> SMEMYETLGKVGEGSYGTVMKCKHKNTGQIVAIKIFYERPEQSVNKIAMREIKFLKQFHHENLVNLIEVFRQKKKIHLVFEFIDHTVLDELQHYCHGLESKRLRKYLFQILRAIDYLHSNNIIHRDIKPENILVSQSGITKLCDFGFARTLAAPGDIYDDEVATRWYRAPELVLKDTSYGKPVDIWALGCMIIEMATGNPYLPSSSDLDLLHKIVLKVGNLSPHLQNIFSKSPIFAGVVLPQVQHPKNARKKYPKLNGLLADIVHACLQIDPADRISSSDLLHHEYFTRDGFIEKFMPELKAKLLQEAKVNSLIKPKESSK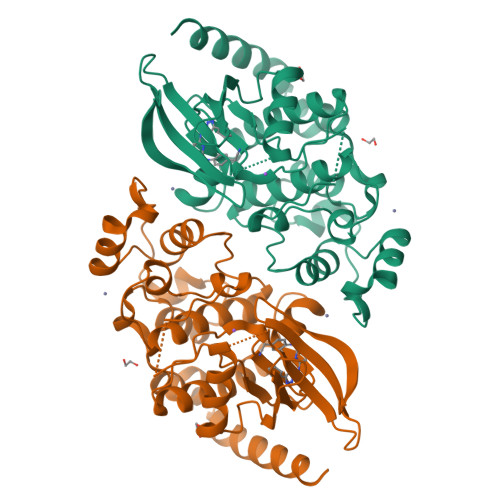ENEL>[2x]DRSRVFDILSNINIGWNLGNTLDATGGGNSVNAETSWGNPKTTQEIVDTVNDRGFNAIRIPVTFANHLGPAPEYTISADWLARVKEVVDYAVNDGMYIILDTHHETNYWLKTDPNNEAALCEELAAIWKQLAEAFKDYDEKLMFEGMNEPRMAG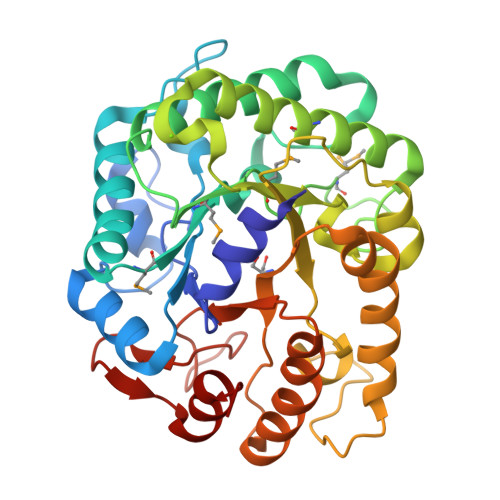SAKEWSGGTPAERKLINAMNKAFIDAVRATGGNNADRVLIICTYGHNSDEPTLKDLEIPSDPNIAVALHTYTPYFFTYVADGSYSVWNGSKKNDITWQYNNIKKYLIDKGIPVVITETGAQFKENTEDIVRWIGDYVGTLDQDGVKCFIWDNNIYHGNGEKFGLLNRSLLKWYNDDIVDAYVNHAA>[2x]MILDTDYITEDGKPVIRIFKKENGEFKIDYDRNFEPYIYALLKDDSAIEDVKKITAERHGTTVRVVRAEKVKKKFLGRPIEVWKLYFTHPQDQPAIRDKIKEHPAVVDIYEYDIPFAKRYLIDKGLIPMEGDEELKMLAFAIATLYHEGEEFAEGPILMISYADEEGARVITWKNIDLPYVDVVSTEKEMIKRFLKVVKEKDPDVLITYNGDNFDFAYLKKRSEKLGVKFILGREGSEPKIQRMGDRFAVEVKGRIHFDLYPVIRRTINLPTYTLEAVYEAIFGQPKEKVYAEEIAQAWETGEGLERVARYSMEDAKVTYELGKEFFPMEAQLSRLVGQSLWDVSRSSTGNLVEWFLLRKAYERNELAPNKPDERELARRRESYAGGYVKEPERGLWENIVYLDFRSLYPSIIITHNVSPDTLNREGCEEYDVAPQVGHKFCKDFPGFIPSLLGDLLEERQKVKKKMKATIDPIEKKLLDYRQRLIKILANSFYGYYGYAKARWYCKECAESVTAWGRQYIETTIREIEEKFGFKVLYADTDGFFATIPGADAETVKKKAKEFLDYINAKLPGLLELEYEGFYKRGFFATKKKYAVIDEEDKITTRGLKMVRRDWSEIAKETQARVLEAILKHGDVEEAVRIVKEVTEKLSKYEVPPEQLVIYQPITKQLHDYRARGPHVSVAKRLAARGIKIRPGTVISYIVPKGSGRIGDRAIPFDEFDPAKHKYDAGYYIENQVLPAVERILRAFGYRKEDLRYQKTRQVGLGAWLKPKT

Archaeal DNA polymerases from the B-family (polB) have found essential applications in biotechnology. Variants of the archaeal polymerase from Thermococcus gorgonarius, TgoT, that can either generate HNA from DNA (TgoT_6G12) or DNA from HNA (TgoT_RT521) have been previously identified. In this study, six X-ray structures of DNA and HNA polymerases are reported: (i) three apo- structures of TgoT, TgoT_6G12, and TgoT_RT521-; (ii) two DNA-bound structures of TgoT_6G12 in binary and ternary complexes; and (iii) one DNA-bound structure of TgoT_6G12, which has incorporated two HNA nucleotides. Consistent with all other DNAPs from B-family, TgoT and its variants fold into five distinct structural subdomains.

In a second experiment, crystals including an incoming nucleotide trapped inside the polymerase active site were generated. The crystals of the ternary complex of TgoT_6G12 diffracted to 3.2 Å, with two molecules per asymmetric unit. However, the thumb region in the ternary complex is mainly ordered. Indeed, only one internal region from amino acid 666 to 690 as well as the C-terminal part from amino acid 763 to the end are poorly defined. Contrary to the structure of TgoT_6G12 in the apo or binary complex, the finger domain of TgoT_6G12 in the ternary complex shows a closed conformation, indicated by a rotation of 24° of its two α-helices (α14 and α15). In the ternary structure of TgoT_6G12, three metal ions are observed at the active site, in the same position as observed with the structure of KOD in ternary complex (Mg2+ in position A, Mn2+ in position B and C). The presence of the two manganese ions was determined by the anomalous signal. The incoming nucleotide (ddTTP) binding site contains two tyrosines: Y494 and Y409. In addition, Y409 forms the bottom of the binding site. ddTTP packs with its sugar moiety against Y409, as previously observed with the dATP in the structure of KOD polymerase ternary complex. In the X-ray ternary complex obtained in the presence of a DNA-DNA duplex, seven of the mutated residues were well defined, which corresponded to V589A, K659Q, E664Q, Q665P, A681S, L704P, and E730G.>GSKEGEYIKLKVIGQDSSEIHFKVKMTTHLKKLKESYAQRQGVPMNSLRFLFEGQRIADNHTPKELGMEEEDVIEVYQEQTGG[2x];>GSGAGEAEERV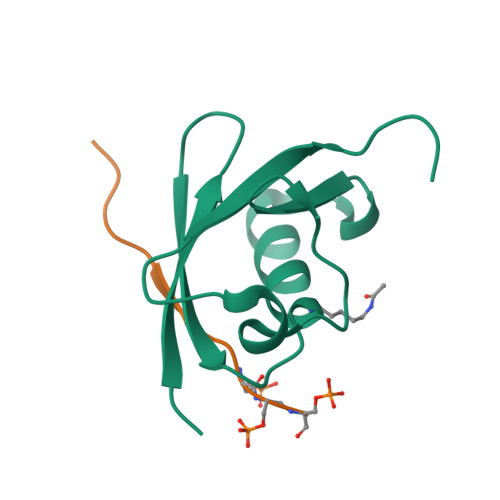VVISSSEDSDAENSSSRY[2x]> TNCD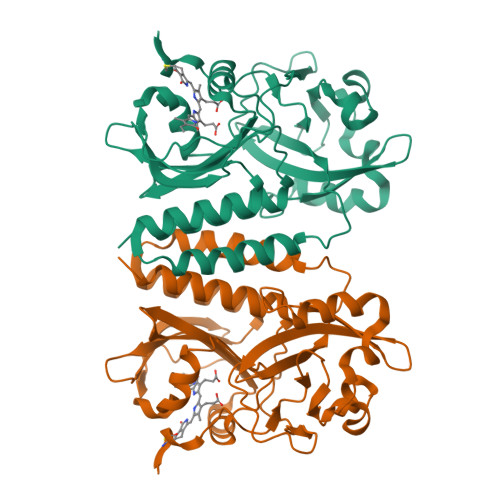REPIHIPGAIQPHGVLLVLSEPGLVLTHASENAPAVLGNSAEQLLGAPLGHFIEPSVREPLEADLRSARLKQLNPLKVVWRVDGVDRFFDGIAHRHQGRLILELEPSSHREAVPFLSFFHAVRDGLSRLRDARDLQELCEAVVQEVRGLTGFDRAIIYRFDAEWNGSVIAEARDARADPYLGLHFPASDIPRQARELYQLNWLRIIPTIDYQPARVRALPGHGEPLDLSFSVLRSVSPIHLEYLHNMGVQASMSISLMKDGKLWGLISCTQVSGTRYVPYEVRTACEFLGEVMSSLLAA>ASSVNELENWSKWMQPIPDNIPLARISIPGTHDSGTFKLQNPIKQVWGMTQEYDFRYQMDHGARIFDIRGRLTDDNTIVLHHGPLYLYVTLHEFINEAKQFLKDNPSETIIMSLKKEYEDMKGAEGSFSSTFEKNYFVDPIFLKTEGNIKLGDARGKIVLLKRYSGSNESGGYNNFYWPDNETFTTTVNQNVNVTVQDKYKVNYDEKVKSIKDTMDETMNNSEDLNHLYINFTS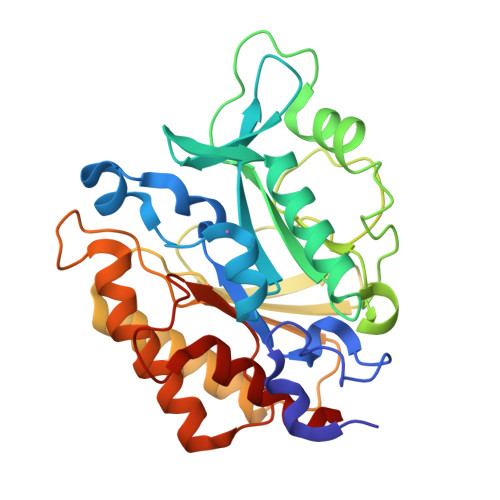LSSGGTAWNSPSSSASSINPEIANDIKQKNPTRVGWVIQDYINEKWSPLLYQEVIRANKSLIKE[2x]> MTNQKFFTLSNGNKIPAVAVVGTGTKWYKAEETDATFSQELTDIVKLSLDTVPGIVHIDAAETYKTYPELGAALKETKKPREEIFITDKFSSLHKISEDPKSAL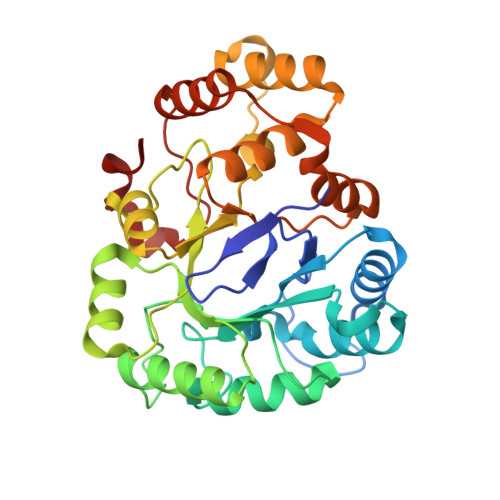ETALNKLGVDYVDLYLIHSPFFDKDLNIDLETAWKQLEELYKSGKAKNIGVSNFTVEDLKKVLAIAEIKPQVNQIEFSPFLQNQTPGIVEFSQKNDILLEAYSPLGPLQKKPTDADQQPFYQYLKELSEKYNKTEAQVLLLWVYKRGILPVTTSAKIERIKQAQDIFSFDLTEEEVKKITDLGLQHEPVRLYHVDFYTKYNSEAQK> GAGMSSPGNSGVAIDSTVLKAIELGTRLFKSGEYLQAKRIFTNALRVCDSYSQE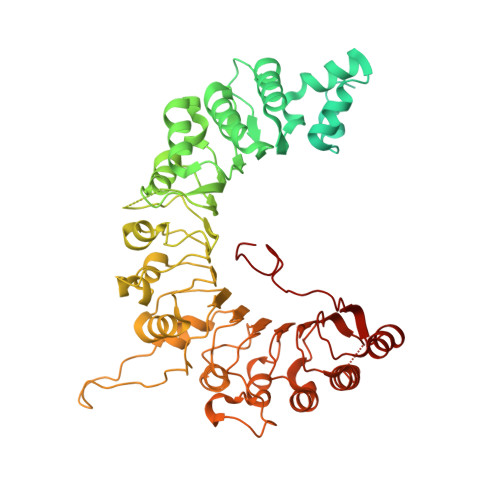QIMRIRNAYQLDTARPDNKRLYHPRYIKILDNICACYEKLNDLKSCLDVSQRLLKLEPGNIKCYIRCTRTLIKLKDWKRAYKTCSRGLQLCNNDSNHLRQQKQFIKNNMVQKQDGKRSYIDPLEETKIAKKKKNNNVLESLPKKKIKGSTKKTDLVGNLPIEILPIIFQRFTTKELVTLSLVCNKWRDKILYHLDCFQEFNLAPINFKNFVKFMDFLQQNFTRTYRKYILSQVKVSSRITSEELRITQLLFSKMPKCINIERLILSMPTLTTTQIFKLMVRGGTDFFTRLLELSLMITYRPDKQHELEILQTCPLLKKIELIFVNSLVPIFDGNNSVGRDGSFNVMARHTNMQISTADNDEQGIVEEKVIYSELEKITLICDKKKIKNFPLCRALLRGQFPLLQKLTITGVTFPMNNQDIMNFQWLLNFPDLKELWIEDNDNCELSKFLQLLKFSNVWKNLEKLTFRENKLYPIVNLDEDQPVTNDDEVPSMLFYKENLQNLEKLDLMGTSISGSALTRLCEQEYLDGRKLRSLNIGNCPNIQFPNNHAHTARMILDVNAVLKRLSKLEEINLSHLSSLNDSTMKSFIINVPFLENLKRLDISHNFEITGISIYEFLKKFQMDHDNEAGGQPLAYLNIDGCSQVSHITVNMIRAQNLVTQVDCVYERDVWRKFGINSYSYS>[2x]RSC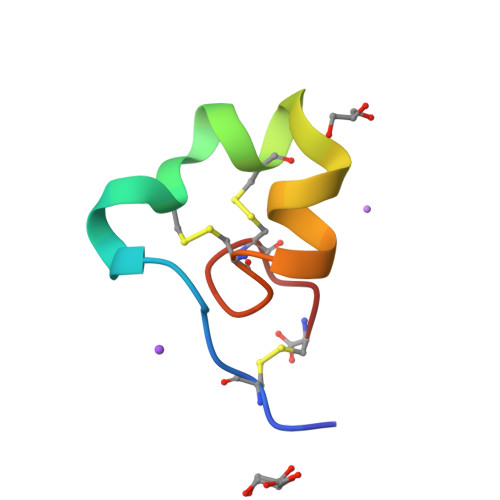IDTIPKSRCTAFQCKHSMKYRLSFCRKTCGTC>MGSSHHHHHHSSGENLYFQGHMRIGIIGLGRMGGNIAVRLTRHGHDVVVHDRTSEVTTSVVGRCEAGRATPADTLADMAKLLEGDEHRVVWVMLPAGAITEDCVQQLGGLLGRGDIIIDGGNTYYKDDVRRSAELAEKGISYVDVGTSGGVWGLERGYCMMFGGTKETAEYIDPILSALAPGIGDVPRTPGRDEAGHDPRAEQGYLHCGPAGSGHFVKMVHNGIEYGMMQAFAEGFDIMKSKNSPILAEKDRFELNMGDIAEVWRRGSVVSSWLLDLTAEALTRSETLNEFSGEVADSGEGRWTIEAAIEED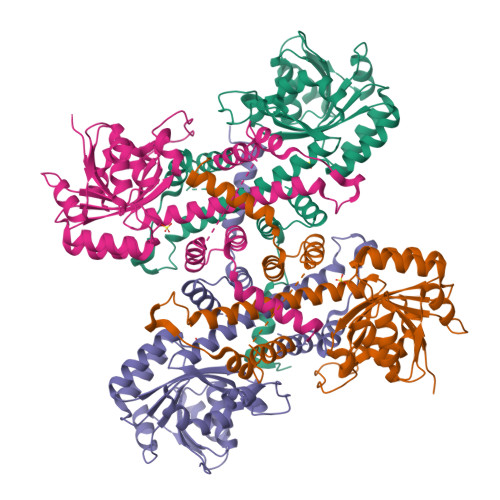VPAPVMTAALFTRFRSRSGNNFAEKILSAQRFGFGGHVEKK[4x]2-methylpropyl N-[(1R)-3-oxidanylidene-1-phenyl-propyl]carbamate | C14 H19 N O3 | 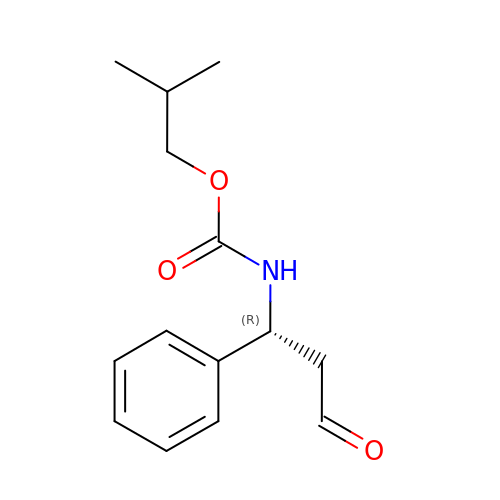DANIFTQCKXMYRY-CYBMUJFWSA-N4-(aminomethyl)aniline | C7 H10 N2 | 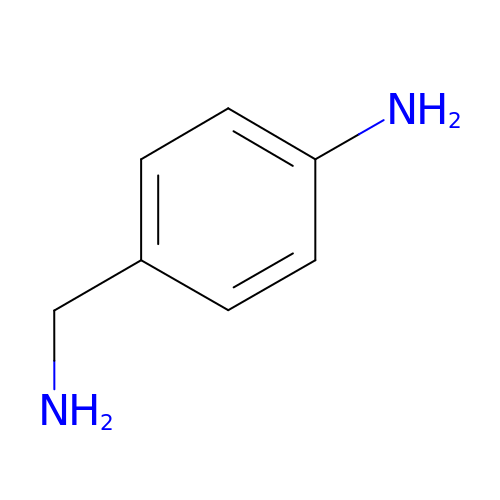BFWYZZPDZZGSLJ-UHFFFAOYSA-N>EPANPNEAYRHYMKKLSYETDIADLSIDIK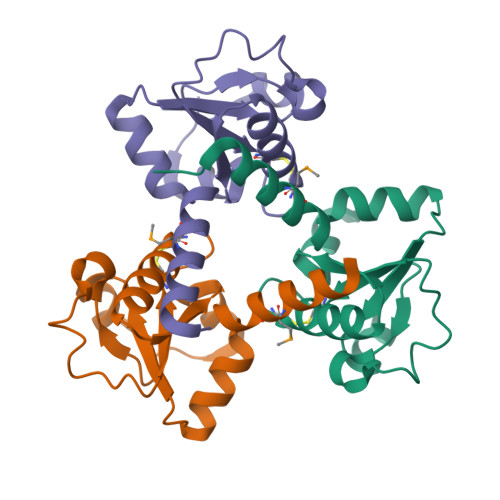KGYEGIIVVDVRDAEAYKECHIPTAISIPGNKINEDTTKRLSKEKVIITYCWGPACNGATKAAAKFAQLGFRVKELIGGIEYWRKENGLEHHHHHH[9x]>GPGYQDPNNRYSFIGGRTGQWQVVKIRNVLGPGLQLVEKVNILNGAVAEIPLDSAWRLQGFASNIRYA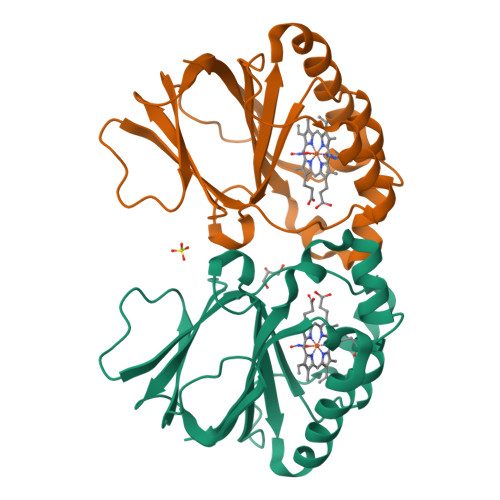IRTELEALQAVQPMLNRAEAILAVLIPIKKSAQWWEMAQDERRDIFERESHHTAVGLEYLPGVARRLLHCRDLGEEFDFLTWFEFAPEHSSAFNELLLRMRASKEWEYVEREVEVWLKRL[2x]>[2x]GSTDITQYEVVEDHNIS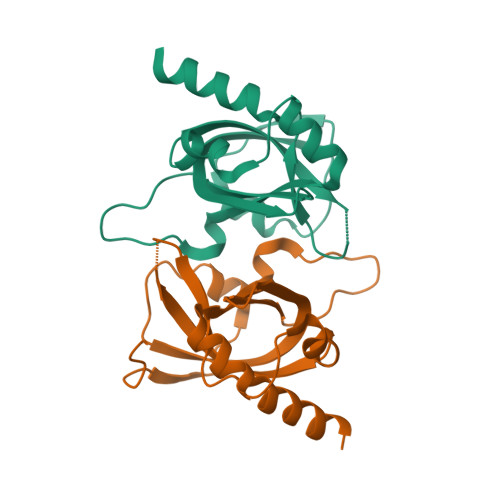QLNHLQHLTPKIYVLNVYIIDVEIVYDQEIRIKVVNELPLVGKYVPPVDILEVYITGKEEVQNFLGDEVLTMDIFTPLLNETSRLRVFQRPSKTDRIIRWSPIECTIQELRLQRMFRLRDTIKVEETLSLTQ>[4x]ARKCSLTGKWTNDLG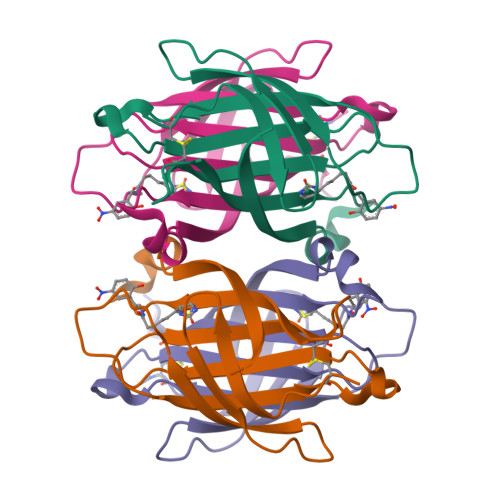SNMTIGAVNSRGEFTGTYTTAVTATSNEIKESPLHGTENTINKRTQPTFGFTVNWKFSESTTVFTGQCFIDRNGKEVLKTMWLLRSSVNDIGDDWKATRVGINIFTRLRTQKE> GAMAAGVKQLADDRTLLMAGVSHDL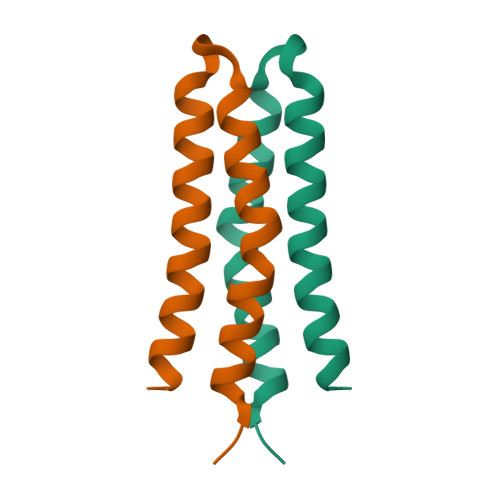RTPLTRIRLATEMMSEQDGYLAESINKDIEECNAIIEQFIDYLR>[13x]MRKFILSLSILLSALLVACSSRNHYGDTGSLAGLQAMADSKYTRAQKKQKMGKIREMALKETALSVGAQAGLAWRAKIIDEQLNKQARNLDAIYDFNSLVLEHNILPPVLLEGRNTLNLADAQSIRISDRTYKVAKQAHFITTPPTWRQYLWMDYVKPEAPNVTLLPKTKAEKEIWCIYTERGWKNGIDQANTILEENIARIKEDFGGMILYRKLLAMNMVSPPYVSHTDLGVTGDGSEIHIDDRVLRITALPELN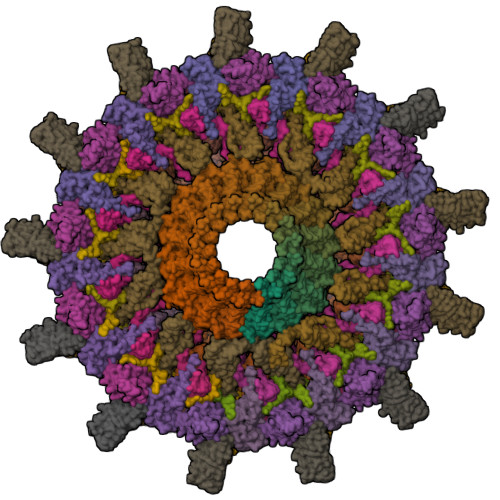VNSAEWRAAVAKDENALERFKNMEKLANQAKIVITNKSWQPIIAPVS;>MNNNKIVIMFIFSALLAGCAGTMKFKKPPINNPSDDATIKLAEAAVSVSDSMLEMAKVEKVITPPSKDNTLTIPNAYNLQARASVDWSGPIEELTARIAKAAHFRFRVLGKSPSVPVLISISTKDESLAEILRDIDYQAGKKASIHVYPNSQVVELRYAKIYS[26x];>[31x]MMAEHDQNNDEYKFAELDSYDMDQAGESDLDSEASYQSGKEGLTKKKDIKRNALIAIGAVVFIMVMYKIIGWMFFSDKSSQVTSKPAIPPVTQVATPQPVQTIPTTTPIQQVQPTTIIEDDPDLKKKVSAIEMTQQSLRSEVNALSEQINAVNNNIKNLNAQIVNLNQIIGNMSNQIARQSEVINVLMARTTPKKVVKVSRPIVQARIIYYIQAVIPGRAWLIGSNGSTLTVREGSKIPGYGMVKLIDSLQGRILTSSGQVIKFSQEDS;>MASKKENLKSLFSNTRTRVIIIFTAALLIIAVVIGFFKIRGATTGSIAAAEVSTVPGGIQSIPGVLDPTAQYAKLQEEQNITQAQVAEKTGGSAIPTIIRTQALGEGVGVIGSQSGVGFAALAQEELGGPQRSLWIQELQDGSCSKSVITKVVNQGAQLTDLKAACSCVQLKDSGYGLQELEQVCECKELKSAGYNARQLKEAGYSAGRLRNCGFDACELRNAGFTAQEMKDGGFSDGELKGAGFSDAEIAKASGLPDGITADDVRKAGCGAAALAKLRQAGVSASAIRKISGCTAEQLKAAGYTAKELKDAGFSAADLRRAGFSAAELKDAGFTARDLLNAGFTPADLAKAGFSDAQIKAAQAELPPGITPQDVKNAGCDVEALKKEREAGVSAALIRQYAGCSAQALKAAGFTDADLANAGFTPAQISAATPLSDAEIKAAGCDPDKLKKLFSAGVSAKRIKELNGCSAEALKAAGYDAQSLLAAGFTPQELLAAGFTPKQLEDAGLNPVSIIADGRVADCSVESLKKARAAGVSALTIKQTLGCSAAALKAAGYTAKELKDAGFTAAELKAAGFSAKELKDAGFTAKELRDAGFSAQELKDVGFSAKDLKDAGFSAAELKAAGFTAAQLKAAGFSAKDLKDAGFSAAELKAAGFSAKELKDAGFSASDLKNAGFSAKELKDAGFSASDLKSAGFSASELKNAGYSADELKKAGYTSAELRNAGFSPQESAVAGLQGPDLQQLDSSITGIPSIPGATPRPTTSDAASSAEQLQAILQKQNEQLAEQKYQQEIQQRTSDMLTAATQLVQDWKQVETQVYTEGTEETKTSGGESAVPGTGTGTGSNNQPVDQGAVSAQNQAIIKTGDIMFAVLDTSVNSDEPGPILATIVTGKLKGSKLIGSFNLPSNADKMVITFNTMSIPGAEKTISISAYAIDPNTARTALASRTNHHYLMRYGSLFASSFLQGFGNAFQSANTTITIGGTGGGNNITVANGVGRSTLENAVIGLATVGKAWSQQAQQLFNTPTTVEVYSGTGLGILFTQDVTTI[34x];>MMKKYDQLCKYCLVIGLTFSMSCSIYAADQSDDAQQALQQLRMLQQKLSQNPSPDAQSGAGDGGDNAASDSTQQPNQSGQANAPAANQTATAGGDGQIISQDDAEVIDKKAFKDMTRNLYPLNPEQVVKLKQIYETSEYAKAATPGTPPKPTATSQFVNLSPGSTPPVIRLSQGFVSSLVFLDSTGAPWPIAAYDLGDPSSFNIQWDKTSNTLMIQATKLYNYGNLAVRLRGLNTPVMLTLIPGQKAVDYRVDLRVQGYGPNAKSMPTEEGIPPSANDLLLHVLEGVPPPGSRRLVVSGGDARAWLSNEKMYVRTNLTILSPGWLASMTSADGTHAYEMQKSPVLLVSWHGKVMQLKVEGL[18x];>[13x]MRSLRTNYIYVLFKTTGLLFLLLLSACNRSGYIPENEVPKLPCRVDGACDATIIKMMTDLNKKGIKVASVGQNYLISIPASALFADQSPRLNWASYSLLNEIAAFLKQFRKIAITVTSYSSKYVSVKRERALTLARSRVVSEYLWSQGVDSRIIFTQGLGSDKPITSYTLGGDRSPNARVEITFRRAVA;>MRNLMRCLIMIKSLIKGVDMSRKLAKTRILGYGLMICFLAGCFHPPYNNFQPDRRAVKRVGVDTGIGAVAGAIASGTASGTLIGAAAGGTVGLVASIYRDSKRKIIRDLQKQDIQYVEYGDTRTLIIPTDKYFMFSSPRLNEICYPGLNNVIRLLNFYPQSTIYVAGFTDNVGSRSHKRKLSQAQAETMMTFLWANGIAAKRLKAEGYGDKNAISDNAIIHGSAQNRRIEIQWFTSPAQPPQPQMAYVK[13x];>[13x]MLKRCYLLILLMFVLASCAHHKPQTPPAEVKKQGTSSTRQFRQVSSFNQIVVQGRLNVNLHTGYNKPEVMLRGDPRDLVQVRTIVKQNTLYVSLGQGYPDYGAVTVDIKTKFLNRFRYEGAGVVTGNNLRTSYLDLYLANEGTTRLAGNIGLQKLEAVGNGVTQINGVSSRNLQIVLKGDPKVLISGFVNLRQLDMYGKGTLSLYWIKSDTLTIRAKKAAKIQLAGIVNRLDVELWDFAQFKGKYLRAQRSFVKTHDKSVAEISAVNHQSSLATDASDIYYYNLSKTRADFMAFNGSVLDMREWGQSDLKDFDRYNKQFP;>MLFLKIKTNQRTTMNILKPKAFLLASVFVLSISPAFAADGCCSKMGGINYCDSSAGRLVCNNGFYSTCYCTRHAVMDLQFLMGCCLWHGGVYPQLNSSGLVVCNDGYVSEECSLQKPVEQISVY[13x]> MDVSGQETDWRSTAFRQKLVSQIEDAMRKAGVAHSKSSKDMESHVFLKAKTRDEYLSLVARLIIHFRDIHNKKSQASVSDPMNALQSLTGGPAAGAAGIGMPPRGPGQSLGGMGSLGAMGQPMSLSGQPPPGTSGMAPHSMAVVSTATPQTQLQLQQVALQQQQQQQQFQQQQQAALQQQQQQQQQQQFQAQQSAMQQQFQAVVQQQQQLQQQQQQQQHLIKLHHQNQQQIQQQQQQLQRIAQLQLQQQQQQQQQQQQQQQQALQAQPPIQQPPMQQPQPPPSQALPQQLQQMHHTQHHQPPPQPQQPPVAQNQPSQLPPQSQTQPLVSQAQALPGQMLYTQPPLKFVRAPMVVQQPPVQPQVQQQQTAVQTAQAAQMVAPGVQMITEALAQGGMHIRARFPPTTAVSAIPSSSIPLGRQPMAQVSQSSLPMLSSPSPGQQVQTPQSMPPPPQPSPQPGQPSSQPNSNVSSGPAPSPSSFLPSPSPQPSQSPVTARTPQNFSVPSPGPLNTPV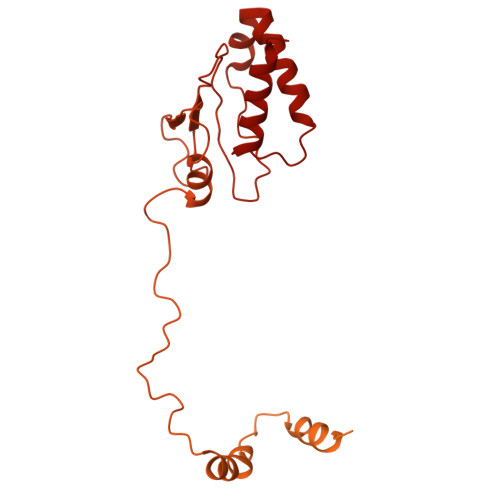NPSSVMSPAGSSQAEEQQYLDKLKQLSKYIEPLRRMINKIDKNEDRKKDLSKMKSLLDILTDPSKRCPLKTLQKCEIALEKLKNDMAVPTPPPPPVPPTKQQYLCQPLLDAVLANIRSPVFNHSLYRTFVPAMTAIHGPPITAPVVCTRKRRLEDDERQSIPSVLQGEVARLDPKFLVNLDPSHCSNNGTVHLICKLDDKDLPSVPPLELSVPADYPAQSPLWIDRQWQYDANPFLQSVHRCMTSRLLQLPDKHSVTALLNTWAQSVHQACLSAA Human gamma-D crystallin (HGD) is a soluble, monomeric protein expressed in the eye lens during fetal development. The high expression levels contribute to the refractive index within the lens which focuses visible light upon the retina. However, this halts further expression of HGD. This means HGD must remain correctly folded and soluble for the entire human lifespan in order to maintain visual acuity. In order to observe structural changes in HGD, we take advantage of an arginine-to-serine point mutation, R36S, first identified in congenital cataracts (HGDm).

The room-temperature serial synchrotron crystallographic (SSX) structure of freshly prepared crystallin mutant (R36S) shows no post-translational modifications. Here, we present crystal structures of freshly prepared HGDm (fresh dataset), HGDm aged for 9 months in dark conditions (aged dataset), and similarly aged HGDm during exposure to UV (light dataset). Crystals were prepared with 20 mM dithiothreitol (DTT), a sulfur-containing reducing agent with a similar function to that which GSH is expected to perform in vivo. In our structures, the fresh HGDm crystals incurred an average diffraction-weighted dose (DWD)28 of 0.19 MGy after 20 ms X-ray exposure. Fo-Fo difference maps calculated between the first and last timepoint revealed no peaks above 3.0 r.m.s.d., confirming that X-ray-induced damage was not responsible for the absence of Cys-DTT in the fresh HGDm structure. The solvent accessibility and pKa of the three surface cysteine residues were calculated from the fresh structure using PropKa331 and PyPka32. Both methods predicted the pKa of C110 to be lower than that of C41 and C108.

>[2x]MKHHHHHHQGKITLYEDRGFQGRHYECSSDHPNLQPYLSRCNSASVDSGCWMLYEQPNYSGLQYFLRRGDYADHQQWMGLSDSVRSCRLIPHSGSHRIRLYEREDYRGQMIEFTEDCSCLQDRFRFNEIHSLNVLEGSWVLYELSNYRGRQYLLMPGDYRRYQDWGATNARVGSLRRVIDFS> AADFDFLKNLSLEELQMRLKALDPMMEREIEELRQRYTAKRQPILDAMDAK;>[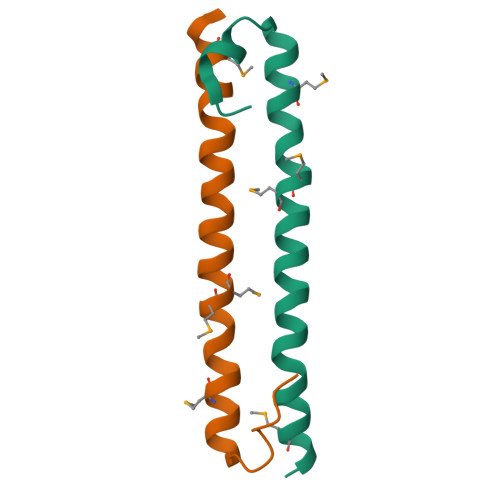3x]DFDFLKNLSLEELQMRLKALDPMMEREIEELRQRYTAKRQPILDAMDAK> XMEAAHSKSTEECLAYFGVSETTGLTPDQVK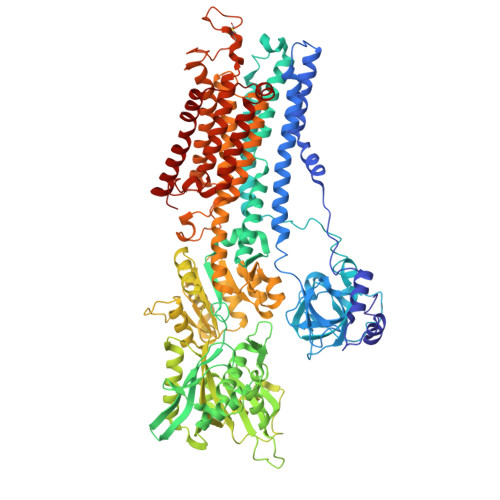RHLEKYGHNELPAEEGKSLWELVIEQFEDLLVRILLLAACISFVLAWFEEGEETITAFVEPFVILLILIANAIVGVWQERNAENAIEALKEYEPEMGKVYRADRKSVQRIKARDIVPGDIVEVAVGDKVPADIRILSIKSTTLRVDQSILTGESVSVIKHTEPVPDPRAVNQDKKNMLFSGTNIAAGKALGIVATTGVSTEIGKIRDQMAATEQDKTPLQQKLDEFGEQLSKVISLICVAVWLINIGHFNDPVHGGSWIRGAIYYFKIAVALAVAAIPEGLPAVITTCLALGTRRMAKKNAIVRSLPSVETLGCTSVICSDKTGTLTTNQMSVCKMFIIDKVDGDFCSLNEFSITGSTYAPEGEVLKNDKPIRSGQFDGLVELATICALCNDSSLDFNETKGVYEKVGEATETALTTLVEKMNVFNTEVRNLSKVERANACNSVIRQLMKKEFTLEFSRDRKSMSVYCSPAKSSRAAVGNKMFVKGAPEGVIDRCNYVRVGTTRVPMTGPVKEKILSVIKEWGTGRDTLRCLALATRDTPPKREEMVLDDSSRFMEYETDLTFVGVVGMLDPPRKEVMGSIQLCRDAGIRVIMITGDNKGTAIAICRRIGIFGENEEVADRAYTGREFDDLPLAEQREACRRACCFARVEPSHKSKIVEYLQSYDEITAMTGDGVNDAPALKKAEIGIAMGSGTAVAKTASEMVLADDNFSTIVAAVEEGRAIYNNMKQFIRYLISSNVGEVVCIFLTAALGLPEALIPVQLLWVNLVTDGLPATALGFNPPDLDIMDRPPRSPKEPLISGWLFFRYMAIGGYVGAATVGAAAWWFMYAEDGPGVTYHQLTHFMQCTEDHPHFEGLDCEIFEAPEPMTMALSVLVTIEMCNALNSLSENQSLMRMPPWVNIWLLGSICLSMSLHFLILYVDPLPMIFKLKALDLTQWLMVLKISLPVIGLDEILKFIARNYLEG>MTVPIAIIGTGIAGLSAAQALTSAGHQVHLFDKSRGSGGRMSSKRSDAGSLDMGAQYFTARDRRFATAVKQWQAQGHVSEWTPLLYNFHGGRLSPSPDEQVRWVGEPGMSAITRAMRGDLPVSFSCRITDVFRGEQHWNLLDAESENHGPFSHVIIATPAPQATALLAAAPKLASVVAGVKMDPTW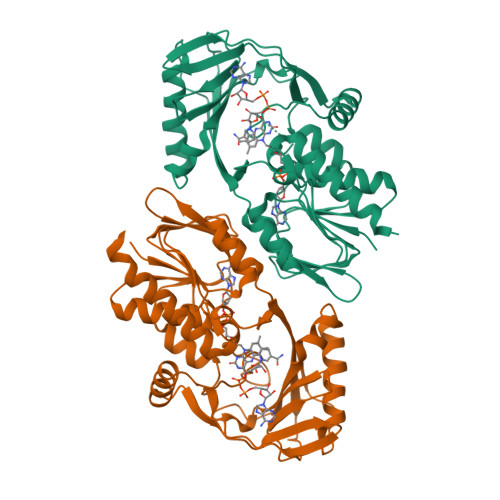AVALAFETPLQTPMQGCFVQDSPLDWLARNRSKPGRDDTLDSWVLHATSQWSRQNLDASREQVIEHLHGAFAELIDCAMPAPVFSLAHRWLYARPAGSHEWGALSDADLGIYVCGDWCLSGRVEGAWLSGQEAARRLLEHLQLEHHHHHH[4x]> ADTIVAVELDSYPNTDIGDPNYPHIGIDIKSIRSKSTARWNMQTGKVGTVHISYNSVAKRLSAVVSYTGSSSTTVSYDVDLNNVLPEWVRVGLSATTGLYKETNTILSWSFTSKLKTNSIADANSLHFTFNQFSQNPKDLIL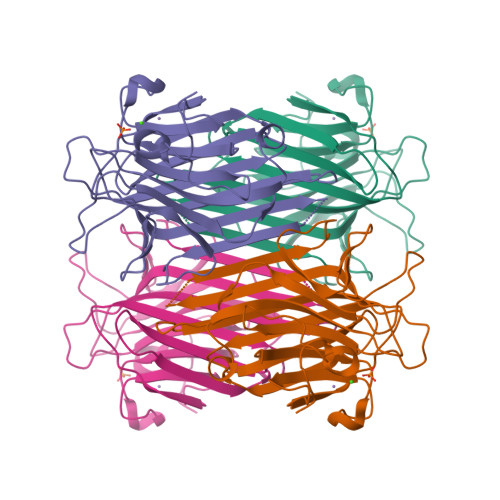QGDATTDSDGNLELTKVSSSGDPQGNSVGRALFYAPVHIWEKSAVVASFDATFTFLIKSPDRDPADGITFFIANPDTSIPSGSGGRLLGLFPDAN> SQE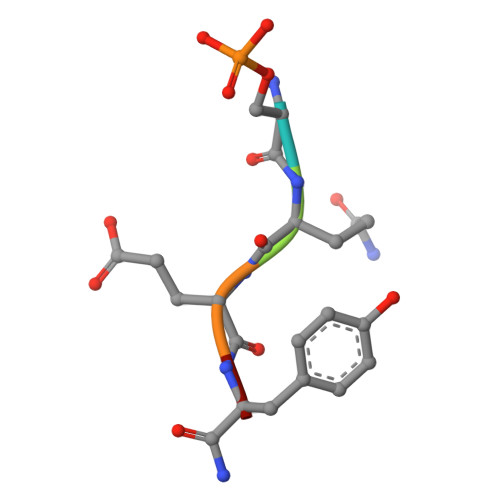YX> ASLTEIEHLVQSVCKSYRETCQLRLEDLLRQRSNIFSREEVTGYQRKSMWEMW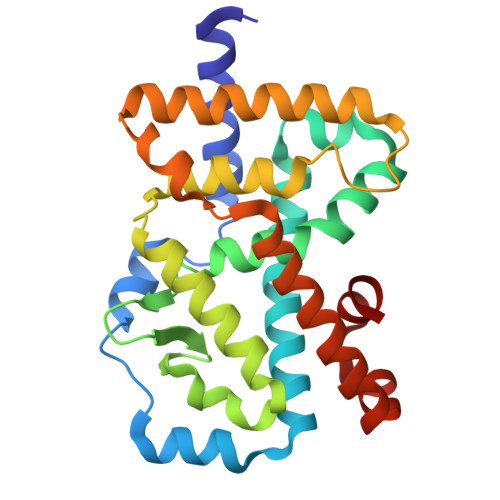ERCAHHLTEAIQYVVEFAKRLSGFMELCQNDQIVLLKAGAMEVVLVRMCRAYNADNRTVFFEGKYGGMELFRALGCSELISSIFDFSHSLSALHFSEDEIALYTALVLINAHRPGLQEKRKVEQLQYNLELAFHHHLCKTHRQSILAKLPPKGKLRSLCSQHVERLQIFQHLHPIVVQAAFPPLYKELFSTE> MASNSPLDEENLTQENQDRGTHVDLGLASANVDFAFSLYKQLVLKAPDKNVIFSPPSISTALAFLSLGAHNTTLTEILKGLKFNLTETSEAEIHQSFQHLLRTLNQSSDELQLSMGNAMFVKEQLSLLDRFTEDAKRLYGSEAFATDFQDSAAAKKLINDYVKNGTRGKITDLIKDLDSQTMMVLVNYIFFKAKWEMPFDPQDTHQSRFYLSKKKWVMVPMMSLHHLTIPYFRDEELSCTVVELKYTGNASALFILPDQDKMEEVEAMLLPETLKRWRDSLE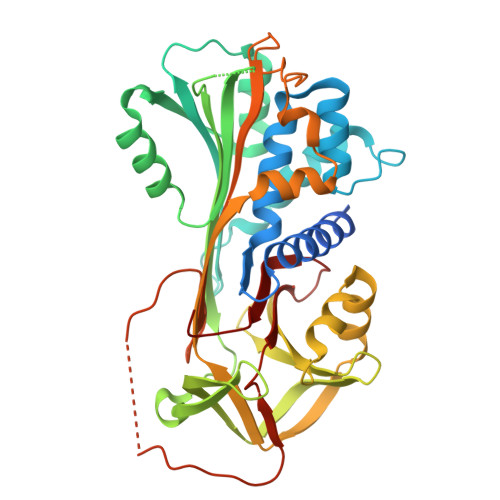FREIGELYLPKFSISRDYNLNDILLQLGIEEAFTSKADLSGITGARNLAVSQVVHKAVLDVFEEGTEASAATAVKITLLSALVETRTIVRFNRPFLMIIVPTDTQNIFFMSKVTNPKQA>MAATTVNGGTVHFKGEVVNAACAVDAGSVDQTVQLGQVRTASLAQEGATSSAVGFNIQLNDCDTNVASKAAVAFLGTAIDAGHTNVLALQSSAAGSATNVGVQILDRTGAALTLDGATFSSETTLNNGTNTIPFQARYFATGAATPGAANADATFKVQYQ[6x];> ADSTITIRGYVRDNGCSVAAESTNFTVDLMENAAKQFNNIGATTPVVPFRILLSPCGNAVSAVKVGFTGVADSHNANLLALENTVSAASGLGIQLLNEQQNQIPLNAPSSALSWTTLTPGKPNTLNFYARLMATQVPVTAGHINATATFTLEYQ

Uropathogenic Escherichia coli strains use filamentous type 1 pili to adhere to and invade uroepithelial cells. The pilus consists of a flexible tip fibrillum, formed by the adhesin FimH and the subunits FimG and FimF. The pilus rod is a helical assembly of up to 3000 copies of the main subunit FimA, terminated by a single copy of the subunit FimI that anchors the rod to the assembly platform FimD in the outer membrane. The assembly platform FimD in the outer membrane of uropathogenic E. coli is the catalyst of type 1 pilus assembly.

We determined the cryo-EM structure of the transition from the last tip fibrillum subunit, FimF, to the first turn of the pilus rod at 3.1 Å resolution. The structure revealed key interactions between FimF and the first three FimA subunits (FimA1, FimA2, and FimA3), which are well-resolved and clearly identifiable. In contrast, the preceding subunit of the tip fibrillum, FimG, appeared flexible and was only visible at lower thresholds, highlighting its dynamic connection to FimF. Specifically, predominantly hydrophobic interactions were found between FimF (complemented with the donor strand of FimA1) and the donor strand of FimA2, while the interfaces of FimF with FimA1 and FimA3 included both hydrophobic contacts and hydrogen bonding. Notably, superimposition of the first three FimA subunits revealed a conformational shift in the βC-βD loop: while solvent-exposed in FimA1 and FimA2, the loop in FimA3 adopts a different conformation that enables interaction with FimF through five additional hydrogen bonds. These interactions are stabilized by hydrogen bonds between Lys35 and Gln36 of FimF with backbone carbonyl oxygens of specific residues in FimA1, including Ala20, Asp60 and Val23. Importantly, the chemical identity of Lys35 and Gln36 is conserved across FimF homologs of other chaperone-usher pili at the transition from the tip fibrillum to the rod. However, Arg38 and Gln36 are shifted by a few residues when aligned to sequences of other FimF homologs, consistent with the substantially different orientation of adjacent FimA rod subunits compared to the FimA-FimF interface. Thus, these differences in the interfaces and the simultaneous interaction of FimF with FimA1, FimA2 and FimA3 are likely incompatible with a FimA-like orientation within the helical rod and thereby facilitate the transition between the linear tip fibrillum and the helical rod architecture. Models of the tip-to-rod transitions in F1C/S pili, F9 pili, P pili, and Yfc pili show that all FimF homologs point upward in a manner similar to FimF. This underlines the critical role of FimF homologs that function as adaptors aligning the tip fibrillum with the axis of the pilus rod.5-acetamido-2,6-anhydro-3,5,9-trideoxy-3-fluoro-D-erythro-L-gluco-non-4-ulosonic 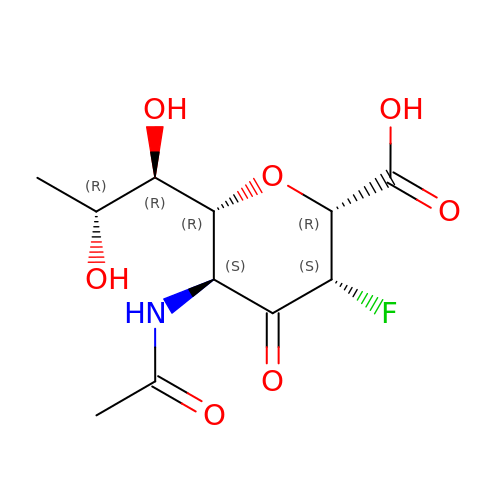acid | C11 H16 F N O7 | CNGWPEUTMWFBNW-QITVGDPKSA-N> MSNLGENKHYEVAKKCVEDLALYLKPLSGGKGVASLNQSALSRPMQRKLVTLVNCQLVEEEGRVRAMRAARSLGERTVTELILQHQNPQQLSANLWAAVRARGCQFLGPAMQEEALKLVLLALEDGSALSRKVLVLFVVQRLEPRFPQASKTSIGHVVQLLYRASCFKVTKRDEDSSLMQLKEEFRSYEALRREHDAQIVHIAMEAGLRISPEQWSSLLYGDLAHKSHMQSIIDKLQSPESFAKSVQELTIVLQRTGDPANLNRLRPHLELLANIDPNPDAVSPTWEQL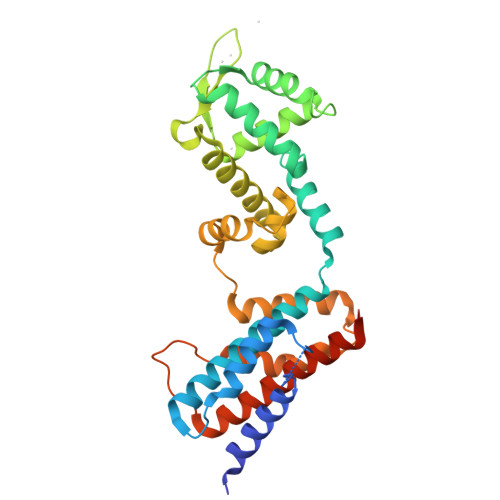ENAMVAVKTVVHGLVDFIQNYSRKGHETPQHHHHHH[(2S,3R,4R,5R)-5-(6-amino-9H-purin-9-yl)-3,4-dihydroxytetrahydrofuran-2-yl]methyl 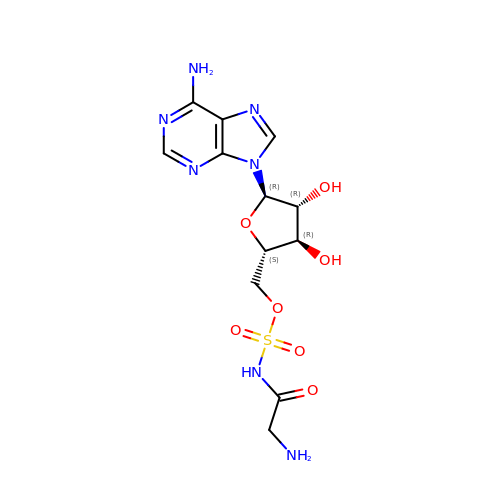(aminoacetyl)sulfamate | C12 H17 N7 O7 S | AMWPZASLDLLQFT-REFFQAGNSA-N>[4x]MKAYKLLTTASIGALMLGMSTAAYSDNWRYAHEEYEGDVQDVFAQA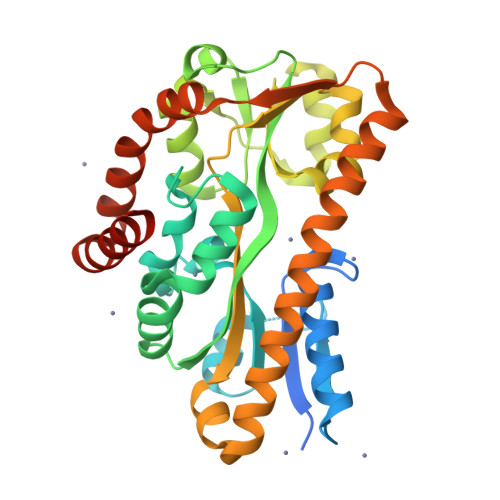FKGYVEDNSDHTVQVYRFGELGESDDIMEQTQNGILQFVNQSPGFTGSLIPSAQIFFIPYLMPTDMDTVLEFFDESKAINEMFPKLYAEHGLELLKMYPEGEMVVTADEPITSPEDFDNKKIRTMTNPLLAETYKAFGATPTPLPWGEVYGGLQTGIIDGQENPIFWIESGGLYEVSPNLTFTSHGWFTTAMMANQDFYEGLSEEDQQLVQDAADAAYDHTIEHIKGLSEESLEKIKAASDEVTVTRLNDEQIQAFKERAPQVEEKFIEMTGEQGQELLDQFKADLKAVQSESEG>NAQFLHTQVGRGLLGAVVNPLGEVTDKFAVTDNSEILYRPVDNAPPLYSERAAIEKPFLTGIKVIDSLLTCGEGQRMGIFASAGCGKTFLMNMLIEHSGADIYVIGLIGERGREVTETVDYLKNSEKK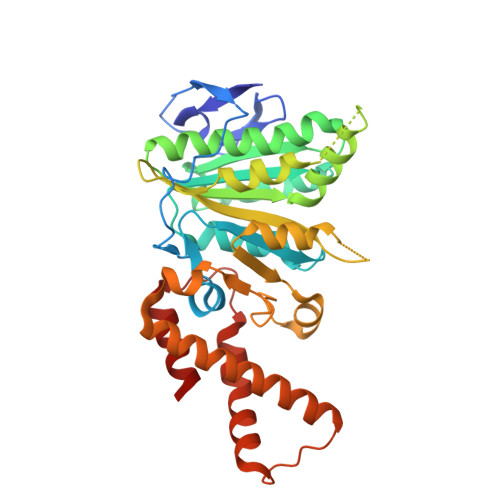SRCVLVYATSDYSSVDRCNAAYIATAIAEFFRTEGHKVALFIDSLTRYARALRDVALAAGESPARRGYPVSVFDSLPRLLRRPGKLKAGGSITAFYTVLLEDDDFADPLAEEVRSILDGHIYLSRNLAQKGQFPAIDSLKSISRVFTQVVDEKHRIMAAAFRELLSEIEELRTIIDFGEYKPGENASQDKIYNKISVVESFLKQDYRLGFTYEQTMELIGETIR[2x]Human strains secrete two papain-like cysteine proteases (staphopains A and B), whereas avian strains express staphopain C (ScpA2). Later findings suggested that ScpA2, as a poultry-specific virulence factor, is directly involved in the pathogenesis of chicken diseases. The X-ray structure of ScpA2 shows the typical fold of the proteases belonging to the papain family. The domains are separated by a V-shaped cleft that contains the active site harboring the conserved catalytic triad (Cys23, His119, Asn140) residues.

In the present study, we determined the three-dimensional crystal structure of ScpA2 at 1.58 Å resolution. Data quality assessment using Xtriage showed that the crystals were tetartohedrally twinned, suggesting a (pseudo)merohedral twinning with four twinned crystal domains. Applying the relevant twinning laws, we found that the crystals belonged to the space group P31 with unit cell parameters of a = b = 103.15 Å and c = 51.21 Å (α = β = 90°, γ = 120°). Three molecules of ScpA2 were found in the asymmetric unit characterized by a solvent content of 54%. The final model of ScpA2 consists of a total of 519 amino acid residues (173 for each monomer), 413 water molecules and 5 chlorine ions. The three molecules in the asymmetric unit are highly similar (root mean square deviation (RMSD) of 0.09 Å). Cys23 forms a thiolate–imidazolium ion pair with His119 (3.5 Å). In ScpA2, the oxyanion hole is composed of two hydrogen bond donors: the Gln17 side chain, and the backbone NH of catalytic Cys23. In staphopain C, the S2 subsite constitutes a hydrophobic pocket lined with Pro66, Met69, Lue95 and Ala117, all of which are conserved among the three best-characterized homologs (ScpA, SspB and ScpA2). This S2 pocket enables the processing of substrates with a hydrophobic side chain at the P2 site, consistent with the information available on the substrate preference of ScpA2.

>[3x]RAQYVNQLKNFKIRETQGNNGWCAGYTMSALLNATYNTDRYNAEAVMRYLHPNLQGDDFQFTGLTPQEMMKYGKSQGRDTQYLNRMPSYNEVDKLTTNNKDIAILGSRVESTDGIHAGHAMAVVGNAELEGGQEVIMIWNPWDRGFMTQDAESNIIPVSNGDHYQWNSSIYGY>[2x]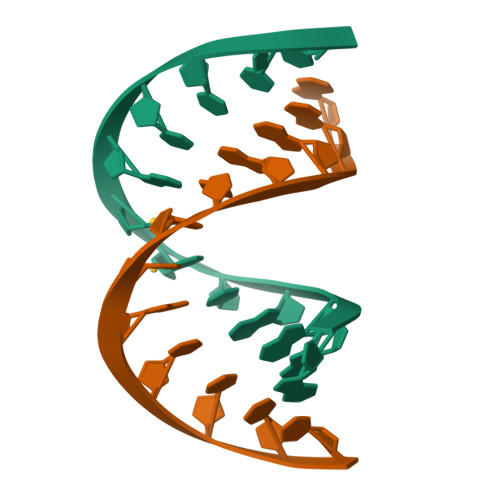GGAGTXXACTCC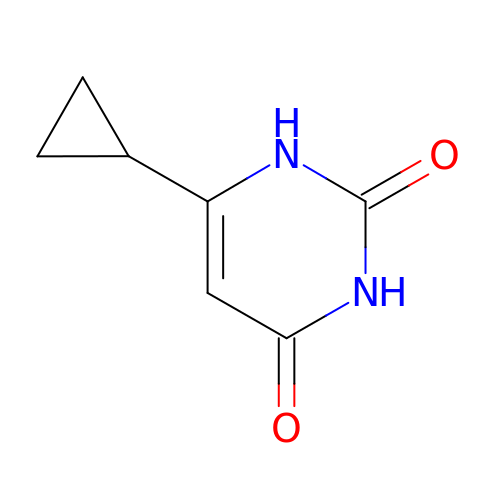6-cyclopropyl-1H-pyrimidine-2,4-dione | C7 H8 N2 O2 | ABHXYFPEQCXJJJ-UHFFFAOYSA-N> M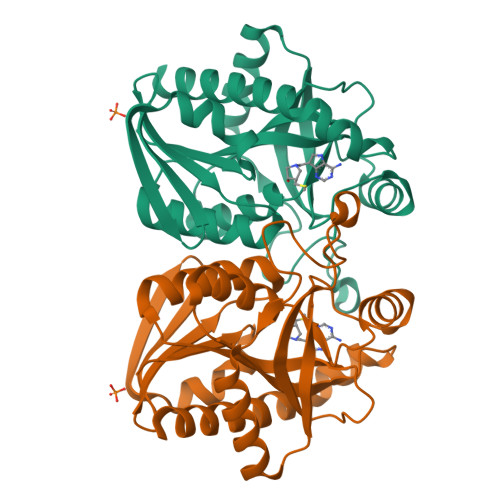KIGIIGAMEEEVTLLRDKIENRQTISLGGCEIYTGQLNGTEVALLKSGIGKVAAALGATLLLEHCKPDVIINTGSAGGLAPTLKVGDIVVSDEARYHDADVTAFGYEYGQLPGCPAGFKADDKLIAAAEACIAELNLNAVRGLIVSGDAFINGSVGLAKIRHNFPQAIAVEMEATAIAHVCHNFNVPFVVVRAISDVADQQSHLSFDEFLAVAAKQSSLMVESLVQKLAHGENLYFQGHHHHHH Among them, levansucrases (sucrose: 2,6-β-d-fructan fructosyltransferase, EC 2.4.1.10) catalyze both sucrose hydrolysis, with the release of glucose and fructose, and levan synthesis. Levansucrase from Bacillus subtilis, Bacillus megaterium, Gluconacetobacter diazotrophicus, Erwinia amylovora, and Erwinia tasmaniensis was extensively purified, and their structure was described. ,− All of them display a single domain with a conserved five-bladed β-propeller topology. ,, Comparison of different levansucrases shows that the architecture of the central substrate-binding pocket is also conserved. In particular, the enzymatic mechanism of sucrose hydrolysis and levan synthesis involves the action of a catalytic triad including two aspartates, acting as a nucleophile and stabilizer, and a glutamate as a general acid/base catalyst. To gain insight into the binding mechanism, the X-ray crystal structures of the beta levansucrase isoform from P. syringae pv actinidiae (Psa) in its native form and in complex with TPIS were solved, confirming TPIS as a competitive inhibitor of levansucrases.

Although X-ray structures of glycosidases in complex with multivalent iminosugars are scarce in the literature − probably due to ligand flexibility, we succeeded in obtaining the crystal structure of Lscβ complexed with TPIS. The binding mode of the pyrrolidine iminosugar in TPIS reflected that previously described for the fructose moiety in the structure of levansucrase mutants of B. subtilis and Brenneria sp. in complex with sucrose. , This confirms that the pyrrolidine iminosugar moiety in TPIS mimics well the fructose moiety in sucrose. In agreement with the competitive mechanism highlighted by kinetic studies, a first binding site was observed at the active site. The hydroxyl groups of one iminosugar unit of TPIS establish hydrogen bonds with the peptide nitrogen of Ala148 and the side chains of catalytic residues Asp219 and Glu303. The endocyclic nitrogen of the same iminosugar unit forms a hydrogen bond with a water molecule that in turn is bound to His113, and a salt bridge with Asp62, considering the nitrogen protonated. The alkyl chain attached to the above-mentioned iminosugar endocyclic nitrogen forms Van der Waals contacts with Trp147, and the ethereal oxygen makes hydrogen bonds with Arg145 and Thr168. The electron density was absent for the remaining part of the tetravalent inhibitor, suggesting a certain degree of disorder relative to the other three iminosugar-ending tails of TPIS, which are likely to occupy multiple conformations. A second molecule of TPIS binds an alternative secondary binding site located at the interface between two different dimers inside the crystal lattice, approximately 30 Å far from the active site.

> MSTSSSALSQLKNSPLAGNINYEPTVWSRADALKVNENDPTTTQPLVSADFPVMSDTVFIWDTMPLRELDGTVVSVNGWSVILTLTADRHPDDPQYLDANGRYDIKRDWEDRHGRARMCYWYSRTGKDWIFGGRVMAEGVSPTTREWAGTPILLNDKGDIDLYYTCVTPGAAIAKVRGRIVTSDQGVELKDFTQVKKLFEADGTYYQTEAQNSSWNFRDPSPFIDPNDGKLYMVFEGNVAGERGSHTVGAAELGPVPPGHEDVGGARFQVGCIGLAVAKDLSGEEWEILPPLVTAVGVNDQTERPHYIFQDGKYYLFTISHKFTYAEGLTGPDGVYGFVGEHLFGPYRPMNASGLVLGNPPEQPFQTYSHCVMPNGLVTSFIDSVPTDGEDYRIGGTEAPTVRIVLKGDRSFVQEEYDYGYIPAMKDVQLS>[4x]MPKRTDIKSILILGAGPIVIGQACEFDYSGAQACKALREEGYRVILVNSNPATIMTDPEMADATYIEPIHWEVVRKIIEKERPDAVLPTMGGQTALNCALELERQGVLEEFGVTMIGATADAIDKAEDRRRFDVAMKKIGLETARSGIAHTMEEALAVAADVGFPCIIRPSFTMGGSGGGIAYNREEFEEICARGLDLSPTKELLIDESLIGWKEYEMEVVRDKNDNCIIVCSIENFDAMGIHTGDSITVAPAQTLTDKEYQIMRNASMAVLREIGVETGGSNVQFAVNPKNGRLIVIEMNPRVSRSSALASKATGFPIAKVAAKLAVGYTLDELMNDITGGRTPASFEPSIDYVVTKIPRFNFEKFAGANDRLTTQMKSVGEVMAIGRTQQESLQKALRGLEVGATGFDPKVSLDDPEALTKIRRELKDAGADRIWYIADAFRAGLSVDGVFNLTNIDRWFLVQIEELVRLEEKVAEVGITGLNADFLRQLKRKGFADARLAKLAGVREAEIRKLRDQYDLHPVYKRVDTCAAEFATDTAYMYSTYEEECEANPSTDREKIMVLGGGPNRIGQGIEFDYCCVHASLALREDGYETIMVNCNPETVSTDYDTSDRLYFEPVTLEDVLEIVRIEKPKGVIVQYGGQTPLKLARALEAAGVPVIGTSPDAI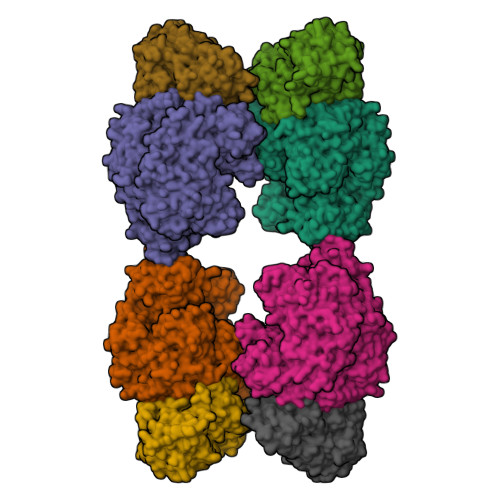DRAEDRERFQHAVERLKLKQPANATVTAIEMAVEKAKEIGYPLVVRPSYVLGGRAMEIVYDEADLRRYFQTAVSVSNDAPVLLDHFLDDAVEVDVDAICDGEMVLIGGIMEHIEQAGVHSGDSACSLPAYTLSQEIQDVMRQQVQKLAFELQVRGLMNVQFAVKNNEVYLIEVNPRAARTVPFVSKATGVPLAKVAARVMAGKSLAEQGVTKEVIPPYYSVKEVVLPFNKFPGVDPLLGPEMRSTGEVMGVGRTFAEAFAKAQLGSNSTMKKHGRALLSVREGDKERVVDLAAKLLKQGFELDATHGTAIVLGEAGINPRLVNKVHEGRPHIQDRIKNGEYTYIINTTSGRRAIEDSRVIRRSALQYKVHYDTTLNGGFATAMALNADATEKVISVQEMHAQIK;>[4x]MIKSALLVLEDGTQFHGRAIGATGSAVGEVVFNTSMTGYQEILTDPSYSRQIVTLTYPHIGNVGTNDADEESSQVHAQGLVIRDLPLIASNFRNTEDLSSYLKRHNIVAIADIDTRKLTRLLREKGAQNGCIIAGDNPDAALALEKARAFPGLNGMDLAKEVTTAEAYSWTQGSWTLTGGLPQAKKEDELPFHVVAYDFGAKRNILRMLVDRGCRLTIVPAQTSAEDVLKMNPDGIFLSNGPGDPAPCDYAITAIQKFLETDIPVFGICLGHQLLALASGAKTVKMKFGHHGGNHPVKDVEKNVVMITAQNHGFAVDEATLPANLRVTHKSLFDGTLQGIHRTDKPAFSFQGHPEASPGPHDAAPLFDHFIELIEQYRKTAK> GSHMTVREQDRFMPIANVIRIMRRILPAHAKISDDSKETIQECVSEYISFITGEANERCQREQRKTITAEDVLWAMSKLGFDDYIEPLTL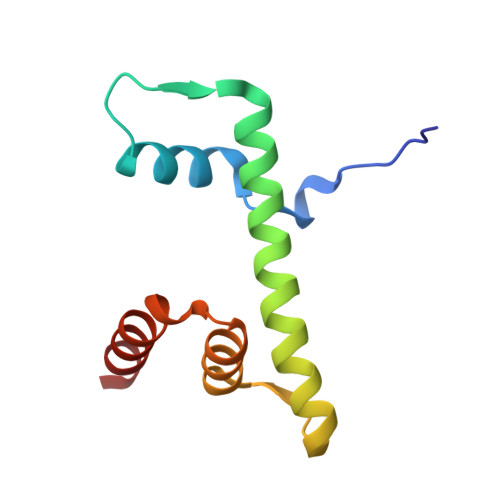YLHRYRE Here we present high performance ultra-low affinity genetically encoded calcium biosensors named GreenT-ECs. GreenT-ECs combine large fluorescence changes upon calcium binding and binding affinities (Kds) ranging from 0.8 mM to 2.9 mM, making them tuned to calcium concentrations in extracellular organismal fluids. The sensors were constructed by inserting a small fragment of a calcium-binding protein (68 amino acids) into a fluorescent protein. Compared to the GCaMP design, prominent in high-affinity biosensors, our design yielded sensors with fewer calcium binding sites per indicator (2 vs 4) and conserved original N-and C-termini of mNeonGreen for the fusion of subcellular targeting motifs.

To elucidate more details on sensor function and for guidance for our protein engineering efforts, we solved a high-resolution crystal structure of an early variant of the sensor in the calcium-bound state to 1.3 A° resolution. It revealed a structure in which the ß-barrel of mNeonGreen is opened to harbor the minimal calcium-binding domain of TnC. Within the TnC domain, the two EF-hand loops with two bound calcium ions and key regions linking the TnC domain to mNeonGreen are visible. Using structure-guided optimization and extended iterative directed evolution we were able to dramatically enhance fluorescence changes and response behavior of the sensors. The binding affinity was drastically reduced by inserting either an additional aspartic acid after position 168 (GreenT-EC) or a serine after position 204 (GreenT-EC.b) within the EF-hand calcium chelating loops.

> MVSKGEEDNMGSLPATHELHIFGSINGVDFDMVGQGSGNPNDGYEELNLKSTKGDLQFSPWILVPHIGYGFHQYLPYPDGMSPFQAAMVDGSGYQVHRTMQFEDGASLTVNYRYTYEGSHIKGEAQVKGTGFPADGPVMTNSLTAADLGWDSEEELSECFRIFDFDGNGFIDREEFGDIIRLTGEQLTDEDVDEIFGDSDTDKNGRIDFDEFLKMVENVQLTDNNRSKKTYPNDKTIISTYKWSYTTGNGKRYRSTAITTYTFAKPMAANYLKNQPMYVFRKTELKHSKTELNFKEWQKAFTD>SNAMTQVYNFSAGPAMLPVEVLRRAQQELRDWHGLGTSVMEVSHRSKEFMQVAEESEKDLRDLLNVPANYKVLFCHGGARAQFAAVPLNLLGDRNSADYVDGGYWAHSAIKEAQKYCTPNVIDVTTHDNGLTGIQPMKQWKLSDNAAYVHYCPNETIDGIAIDEQPDFGNKVVVADFSSSILSRPIDVSRYGVIYAGAQKNIGPAGLTLVIVREDLLGKAHTALPSILDYKILADNDSMFNTPPTFAWYLSGLVFKWLKEQGGLGEMEKRNQAKAELLYGAIDRTGFYRNDVAITNRSWMNVPFQMADASLDKLFLSEAEAQGLQALKGHRVAGGMRASIYNAMPIEGVKALTDFMAD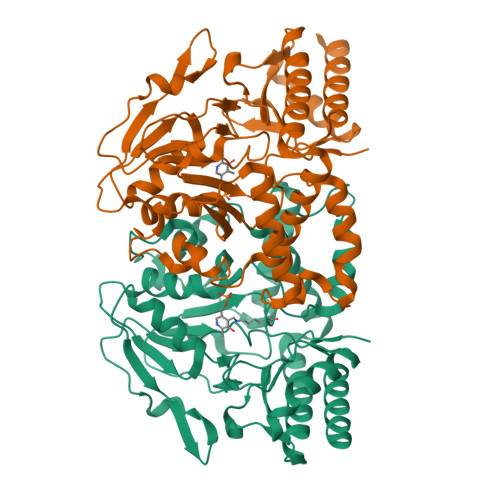FERRHG[2x]> MDQKAIVLDNSKSGSKQTKSSGKMQTQTDTNAEVLNTDNSIKKETGSDSEDLFNKFSNKKTNRKIPNIAEELAKNRNYVKGASPSPIIISGSSSTSPSGPSSSSTNPMGIPTNRFNKNTVELYQHSPSPVMTTNKTDTEEKRQNNRNMDNKNTPERGSSSFAAKQLKISSLLTISSNEDSKTLHINDTNGNKNSNAASNNIPSAYAELHTEGNSIESLIKPPSSPRNKSLTPKVILPTQNMDGTIAKDPHLGDNTPGILIAKTSSPVNLDVESTAQSLGKFNKSTNSLKAALTKAPAEKVSLKRSISSVTNSDSNISSSKKPTSEKAKKSSSASAILPKPTTTKTSKKAASNSSDSTRKKNASNKTTSAIKKESNAGSKLNTVKKENSSLSSIKATEKEKDKGGNSTEAKNSTSNVRKEPTAKSPKRLVAAPTVSPPKILQTAETKAKEPSILIDVPLYQADTNDYLDENGQVIFNLSTLIKEKYHPKSKELAQLKDSKRNLLMQLSDHSNGSLEKEKDEEGDVIELDDDEDMEEDEGEIDTETNTVTTTISPKKKSHPMKGKNLIGKYDVEDPFIDDSELLWEEQRAATKDGFFVYFGPLIEKGHYASLERANGTMKRGGVK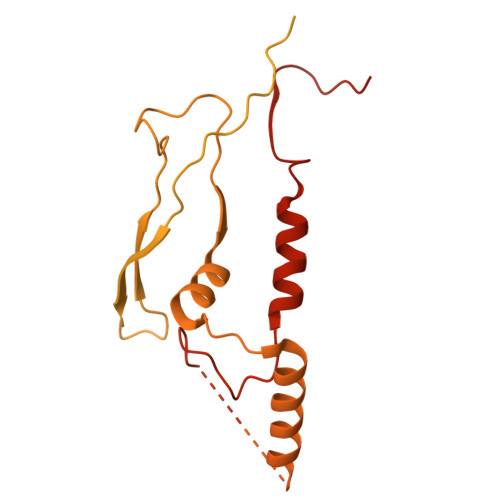NK>[14x]GSHMQMVPPSAYDRAITVFSPEGRLYQVEYAREAVRRGTTAIGIACKDGVVLAVDRRITSKLVKIRSIEKIFQIDDHVAAATSGLVADARVLIDRARLEAQIYRLTYGEEISIEMLAKKICDIKQAYTQHGGVRPFGVSLLIAGIDKNEARLFETDPSGALIEYKATAIGS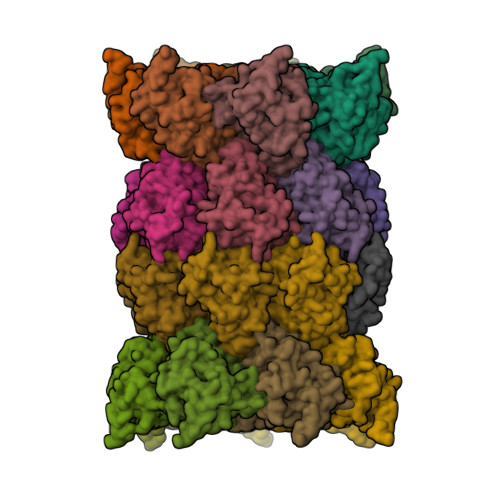GRPVVMELLEKEYRDDITLDEGLELAITALTKANEDIKPENVDVCIITVKDAQFKKIPVEEIKKLIEKVKKKLNEENKKEEENREETKEKQEE;>MTTTVGLICDDAVILATDKRASLGNLVADKEAKKLYKIDDYIAMTIAGSVGDAQAIVRLLIAEAKLYKMRTGRNIPPLACATLLSNILHSSRMFPFLTQIIIGGYDLLEGAKLFSLDPLGGMNEEKTFTATGSGSPIAYGVLEAGYDRDMSVEEGIKLALNALKSAMERDTFSGNGISLAVITKDGVKIFEDEEIEKILDSMKAKPKKKTTKRSRRKSK[14x]> DRHHHHHHKLSYSLSGSWRVSNGNGSLELPATVPGYVHSALHQHGLIQDPYYRFNDLNYRWISLDNWTYSTEFKIPFNLSEWQKVKLIFDGVDTVAEILFNNVTIGKTDNMFTGYSFDITNVVKDVNSLKLQFRSAVQYAECQSKAHTSYRVPPECPPVEQKGECHVNFIRKAQCSFSWDWGPSFPSQGIWKDVRIEAYNIAHLDYLTFLPVYDNASQAWNIEIKASFDVASSKSVGGQVTVAIPQLKTQQTNDIELQQEQRIVKLLVKIRKDVAVETWWPRGHGNQTGYNMTILFALDGGLKIEKAAKVYFRTVQLIEEGIKGSPGLSFYFKINGLPIFLKGSNWIPADSFQDKVTSDRLQLLFQSVVDANMNTLRVWGGGIYEQDEFYALCDELGIMVWQDFMFASALYPTEPGFLASVRKEVTYQVRRLKSHPSIIIWSGNNENEVALSVNWFHVNPRDMKTYIDDYVTLYVKNIRKIVLSE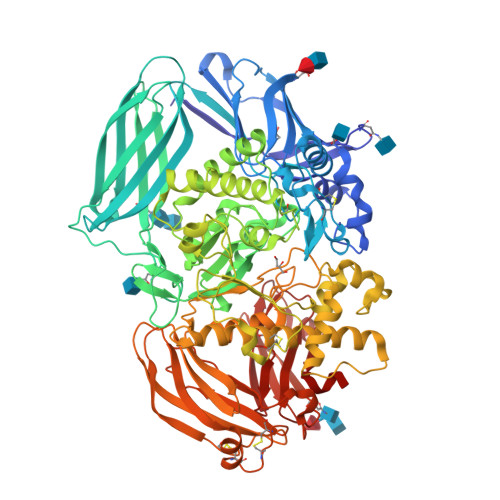DKSRPFIASSPTNGMKTMEEGWISYDPYSIQYGDIHFYNYADDCWNWKIFPKARLVSEYGYQSWPSFSTLEKVSSQEDWAYNSRFSLHRQHHEDGNHQMLHQVKMHFKLPQGTDPLRTFKDTIYLTQVMQAQCIKTETEFYLRSRSEIVDGKGHTMGALYWQLNDIWQAPSWASLEYGGKWKMLHYFARRFFAPLLPVGFEDEGVFYVYGVSDLHKDHHTQLTVRLHHWSSPKPLCSLVNSSIVVKAGEAVVLFQMPVSELLKRCRGCTRETCVVSFYFSTDKELFSPTNYHFLSSLKDAKGLLEANITVNISQKGNVFVFDLETSAVAPFVWLDVGSIPGRFSDNGFLMIRKKLSVLFYPWKPTSKSELQQAFSVTSLTDTY>AGFCEVCEKLVGYLDRNLEKNSTKQEILAALEKGCS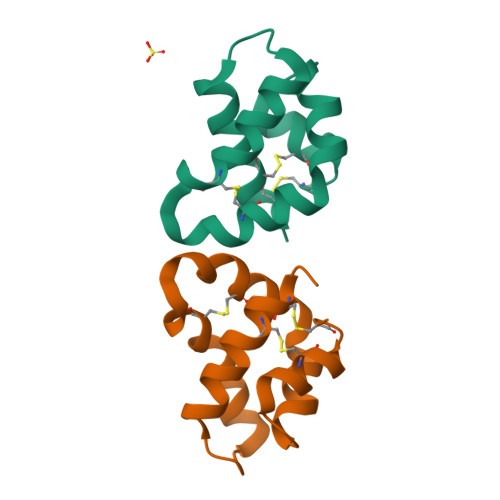FLPDPYQKQCDQFVAEYEPVLIEILVEVMDPSFVCLKIGACPSHHHHHH[2x]> MGSSHHHHHHSQDPNSASLPGIDEHTTSEELITGDNEWHKLVIPKGSDWQIDLKAEGKLIVKVNSGIVEIFGTELAVDDEYTFQNWKFPIYAVEETELLWKCPDLTTNTITVKPNHTMKYIYNLHFMLEKIRMSNFEGPRVVIVGGSQTGKTSLSRTLCSYALKFNAYQPLYINLDPQQPIFTVPGCISATPISDILDAQLPTWGQSLTSGATLLHNKQPMVKNFGLERINENKDLYLECISQLGQVVGQRLHLDPQVRRSGCIVDTPSISQLDENLAELHHIIEKLNVNIMLVLCSETDPLWEKVKKTFGP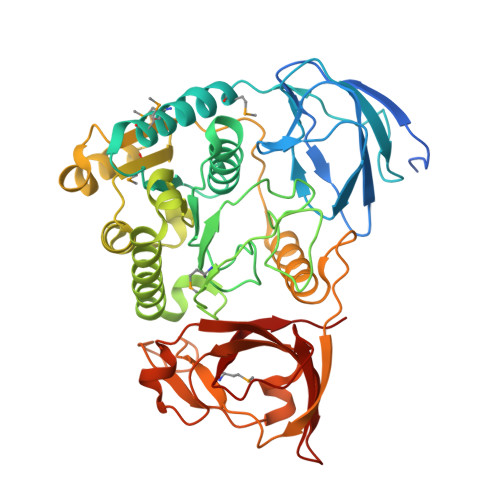ELGNNNIFFIPKLDGVSAVDDVYKRSLQRTSIREYFYGSLDTALSPYAIGVDYEDLTIWKPSNVFDNEVGRVELFPVTITPSNLQHAIIAITFAERRADQATVIKSPILGFALITEVNEKRRKLRVLLPVPGRLPSKAMILTSYRYLE5-(4-tert-butylphenyl)-1-[4-(propan-2-yloxy)phenyl]-1H-indole-2-carboxylic 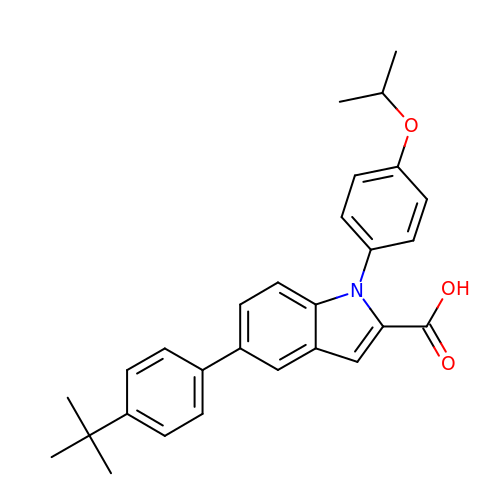acid | C28 H29 N O3 | GUMCVDVWBMLUSQ-UHFFFAOYSA-N> SKMSDVKCTSVVLLSVLQQLRVESSSKLWAQCVQLHNDILLAKDTTEAFEKMVSLLSVLLSMQG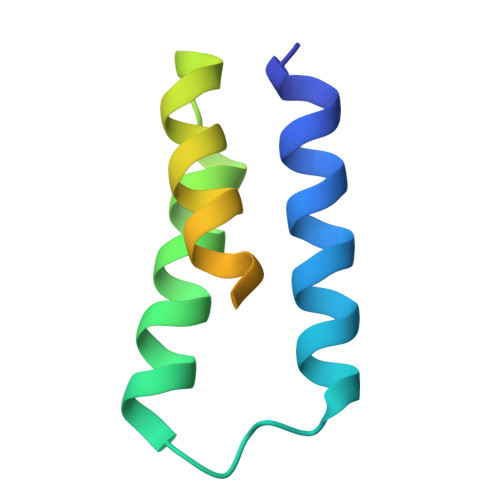AVDINKLCEEMLDNRATLQ>MHHHHHHLEPPPSTFQPLCHPLVEEVSKEVDGYFLQHWNFPNE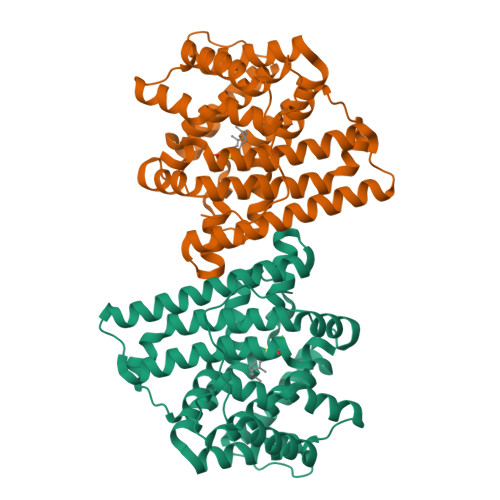KARKKFVAAGFSRVTCLYFPKALDDRIHFACRLLTVLFLIDDLLEYMSFEEGSAYNEKLIPISRGDVLPDRSIPVEYIIYDLWESMRAHDREMADEILEPVFLFMRAQTDRTRARPMGLGGYLEYRERDVGKELLAALMRFSMGLKLSPSELQRVREIDANCSKHLSVVNDIYSYEKELYTSKTAHSEGGILCTSVQILAQEADVTAEAAKRVLFVMCREWELRHQLLVARLSAEGLETPGLAAYVEGLEYQMSGNELWSQTTLRYSVVVD[4x]>ESHMAMDLGGYLTRIGLDGRPRPDLGTLHAIVAAHNRSIPFENLDPLLGIPVADLSAEALFAKLVDRRRGGYQYEHNGLLGYVLEELGFEVERLSGRVVWMRADDAPLPAQTHNVLSVAVPGADGRYLVDVGFGGQTLTSPIRLEAGPVQQTRHEPYRLTRHGDDHTLAAQVRGEWQPLYTFTTEPRPRIDLEVGSWYVSTHPGSHFVTGLTVAVVTDDARYNLRGRNLAVHRSGATEHIRFDSAA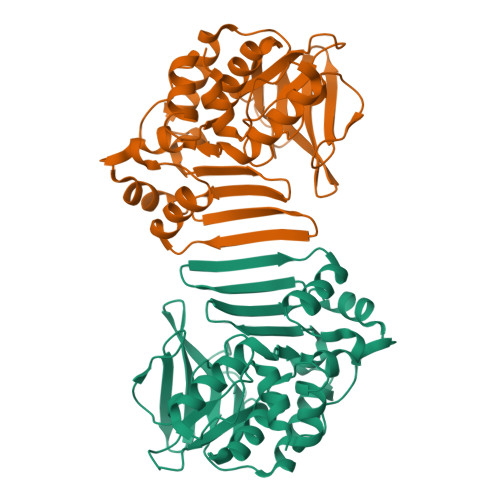QVLDAIVNRFGIDLGDLAGRDVQARVAEVLDT[2x]> SSIMTSENHLNNSDKEVDEVDAALSDLEITLEGGKTSTILGDITSIPELADYIKVFKPKKLTLKGYKQYWCTFKDTSISCYKSKEESSGTP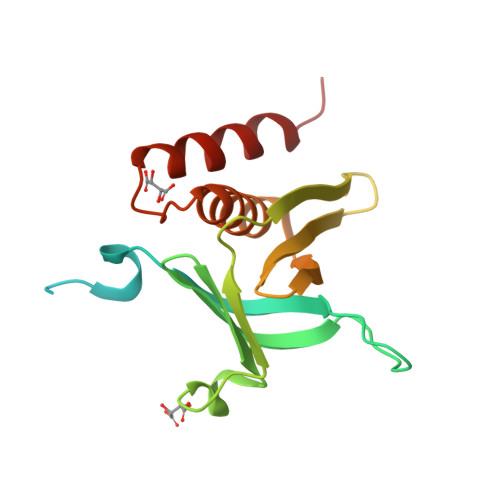AHQMNLRGCEVTPDVNISGQKFNIKLLIPVAEGMNEIWLRCDNEKQYAHWMAACRLASKGKTMADSSYNLEVQNILSFLKMQ> HHHHHHEVLLRSTETGQWLRINPDGTVDGTRDRSDPGIQWQISPEGNGEVLLRSTETGQWLRINPDGTVDGTRDRSDPGIQWQISPEGNGEVLLRS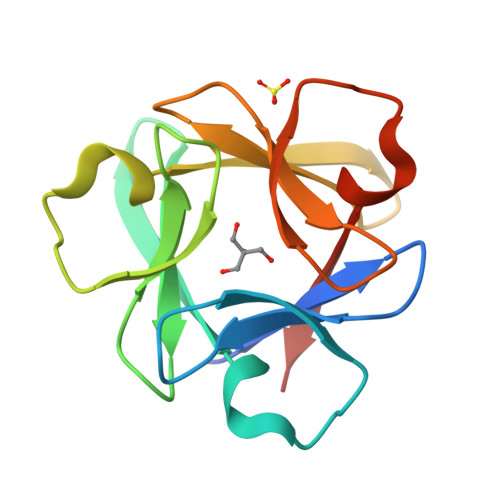TETGQWLRINPDGTVDGTRDRSDPGIQWQISPEGNG>[4x]SMPVRRVRVVKQEAGGLGISIKGGRENRMPIL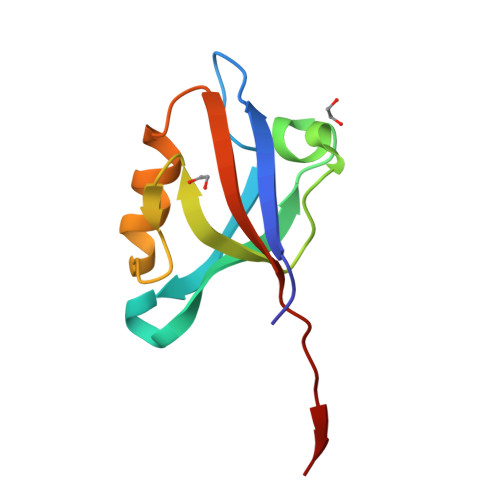ISKIFPGLAADQSRALRLGDAILSVNGTDLRQATHDQAVQALKRAGKEVLLEVKFIREVNTVV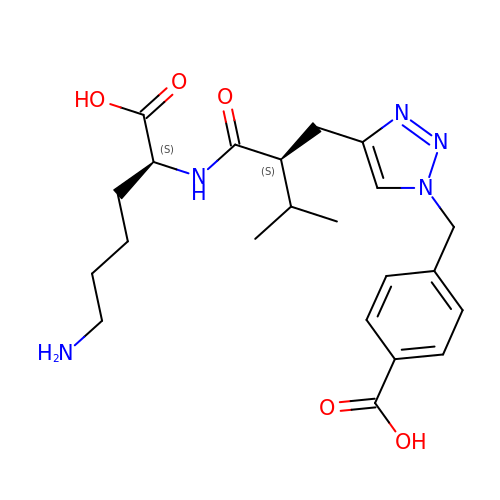N~2~-[(2S)-2-{[1-(4-carboxybenzyl)-1H-1,2,3-triazol-4-yl]methyl}-3-methylbutanoyl]-L-lysine | C22 H31 N5 O5 | ZFYKXBBWZOQIRM-OALUTQOASA-N3-(propylsulfanyl)propyl alpha-D-mannopyranoside | C12 H24 O6 S | 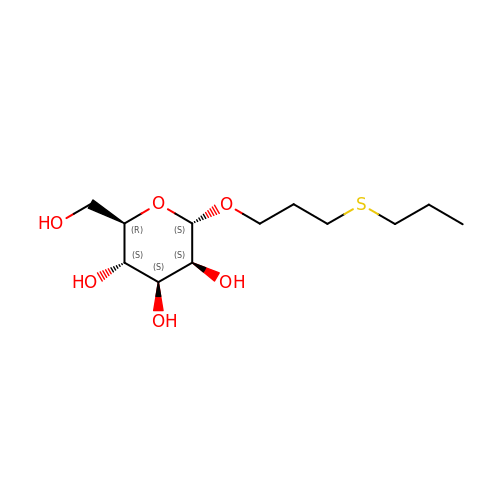VPHBOBPNUZWASC-GCHJQGSQSA-N>GPASPPLLRCLVLTGFGGYDKVKLQSRPAAPPAPGPGQLTLRLRACGLNFADLMARQGLYDRLPPLPVTPGMEGAG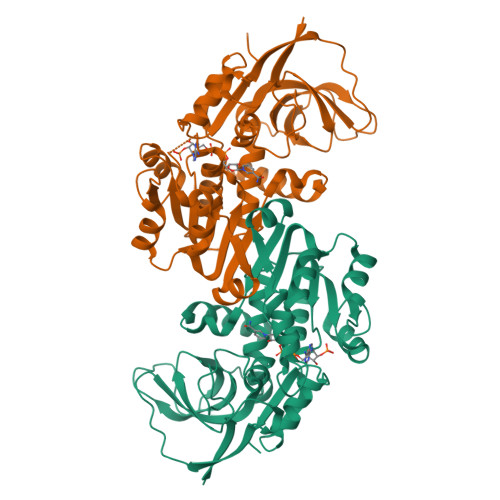VVIAVGEGVSDRKAGDRVMVLNRSGMWQEEVTVPSVQTFLIPEAMTFEEAAALLVNYITAYMVLFDFGNLQPGHSVLVHMAAGGVGMAAVQLCRTVENVTVFGTASASKHEALKENGVTHPIDYHTTDYVDEIKKISPKGVDIVMDPLGGSDTAKGYNLLKPMGKVVTYGMANLLTGPKRNLMALARTWWNQFSVTALQLLQANRAVCGFHLGYLDGEVELVSGVVARLLALYNQGHIKPHIDSVWPFEKVADAMKQMQEKKNVGKVLLVPGPEKEN[4x]2-cyano-~{N}-cyclohexyl-ethanamide | C9 H14 N2 O | 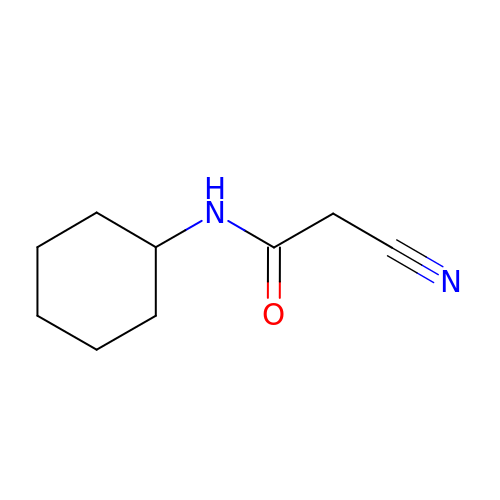RURWLUVLDBYUEN-UHFFFAOYSA-N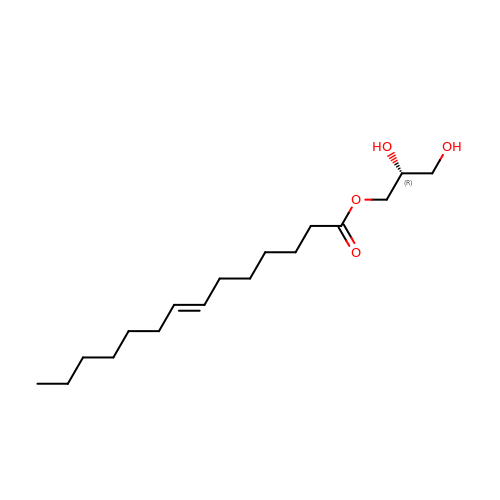(2R)-2,3-DIHYDROXYPROPYL (7Z)-TETRADEC-7-ENOATE | C17 H32 O4 | LVBAGTJIDOCNIJ-XITLMJRVSA-N> X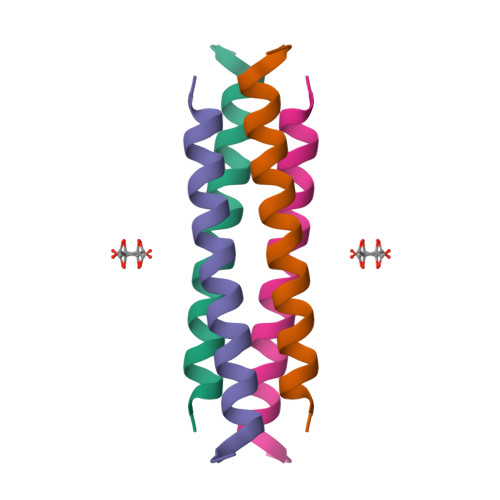GKLEAIAQKLEAIAKKLEAIAWKLEAIAQGAGX> SLAKSAANKLDWAKVISSLRITGSTATQLSSFKKRNDEARRQLLELQSQPTEVDFSHYRSVLKNTSVIDKIESYVKQYKPVKIDASKQLQVIESFEKHAMTNAKETESLVSKELKDLQSTLDNIQSARPFDELTVDDLTKIKPEIDAKVEEMVKKGKWDVPGYKDRFGNLNVM;> MPQLVPFYFMNQLTYGFLLMITLLILFSQFFLPMILRLYVSRLFISKL;> MLKRFPTPILKVYWPFFVAGAAVYYGMSKAADLSSNT;>MQLVLAAKYIGAGISTIGLLGAGIGIAIVFAALINGVSRNPSIKDTVFPMAILGFALSEATGLFCLMVSFLLLFGV[10x];> VSTLIPPKVVSSKNIGSAPNAKRIANVVHFYKSLPQGPAPAIKANTRLARYKAKYFDGDNASGKPLWHFALGIIAFGYSMEYYFHLRHHKGAEEH;> SPLDQFEIRTLFGLQSSFIDLSCLNLTTFSLYTIIVLLVITSLYTLTNNNNKIIGSRWLISQEAIYDTIMNMTKGQIGGKNWGLYFPMIFTLFMFIFIANLISMIPYSFALSAHLVFIISLSIVIWLGNTILGLYKHGWVFFSLFVPAGTPLPLVPLLVIIETLSYFARAISLGLRLGSNILAGHLLMVILAGLTFNFMLINLFTLVFGFVPLAMILAIMMLEFAIGIIQGYVWAILTASYLKDAVYLH;> MSSTPEKQTDPKAKANSIINAIPGNNILTKTGVLGTSAAAVIYAISNELYVINDESILLLTFLGFTGLVAKYLAPAYKDFADARMKKVSDVLNASRNKHVEAVKDRIDSVSQLQNVAETTKVLFDVSKETVELESEAFELKQKVELAHEAKAVLDSWVRYEASLRQLEQRQLAKSVISRVQSELGNPKFQEKVLQQSISEIEQLLSKLK

The F1Fo ATP synthase (M.W. ≈ 600 kDa for the monomer) is highly conserved from bacteria to mammals. The ATP synthase comprises a catalytic F1 portion, a peripheral stalk or stator, and the membrane embedded, Fo region. Fo contains a ring of c-subunits (eight in mammals, ten in yeast, 14 in chloroplast, and various stoichiometries in bacteria) that functions as a proton turbine, along with a-subunit that provides the conduits for proton entry and exit. The c-ring, connected to the central stalk of F1, rotates driven by the movement of protons down the potential gradient from the cytosol of the cell to the mitochondrial matrix, and the proton flow provides the energy for the phosphorylation of ADP in the active site of F1.

We used single-particle cryo-EM to identify the binding site for BDQ on the yeast F1Fo ATP synthase. This analysis was performed essentially using purified enzyme reconstituted into nanodiscs made from palmitoyl-oleoyl-phosphatidylcholine (POPC) and cardiolipin (cardiolipin is 12% by weight). To improve the Fo structure, we reprocessed the cryo-EM data starting from particle picking at the center of Fo, instead of F1Fo. This strategy generated an improved cryo-EM reconstruction of Fo at an overall resolution of 4.2 Å, which is of good quality with side-chain densities visible for many residues. A unique and strong cryo-EM density is clearly observed at the interface between the a- and c-subunits, whose size and shape are consistent with those of a BDQ molecule. The binding of BDQ disrupted the interface between the a- and c-subunits as compared to the reference structures. Helices 5 and 6 of subunit-a are distorted around the proposed binding site of BDQ which increases the space between subunit-a and the c10-ring. Pointedly, aMet215 moves by about 3 Å from the reference structures. The side chain of aMet215 is on the face of the helix closest to the BDQ molecule, and would clash with the EM density of BDQ if it was in the reference conformation. For instance, the phenyl ring of cPhe55 is displaced by as much as 3.1 Å and accompanied by distortion of the α-helix. The cation-π interaction between the t-amine of BDQ and cPhe64 is likely to be a critical interaction that stabilizes BDQ binding.>[2x]MGKRAAHIGLRALADLATPMAVRVAATLRVADHIAAGHRTAAEIASAAGAHADSLDRLLRHLVAVGLFTRDGQGVYGLTEFGEQLRDDHAAGKRKWLDMNSAVGRGDLGFVELAHSIRTGQPAYPVRYGTSFWEDLGSDPVLSASFDTLMSHHLELDYTGIAAKYDWAALGHV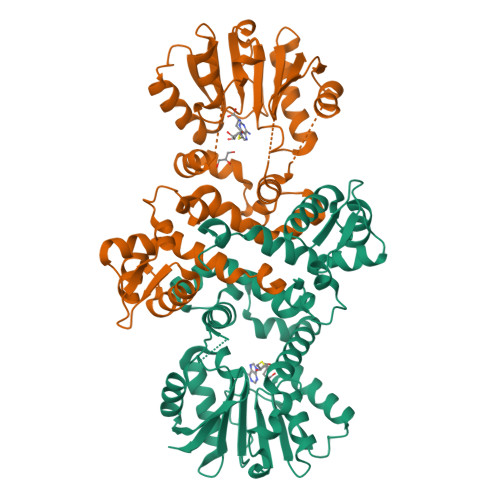VDVGGGSGGLLSALLTAHEDLSGTVLDLQGPASAAHRRFLDTGLSGRAQVVVGSFFDPLPAGAGGYVLSAVLHDWDDLSAVAILRRCAEAAGSGGVVLVIEAVAGDEHAGTGMDLRMLTYFGGKERSLAELGELAAQAGLAVRAAHPISYVSIVEMTAL>[2x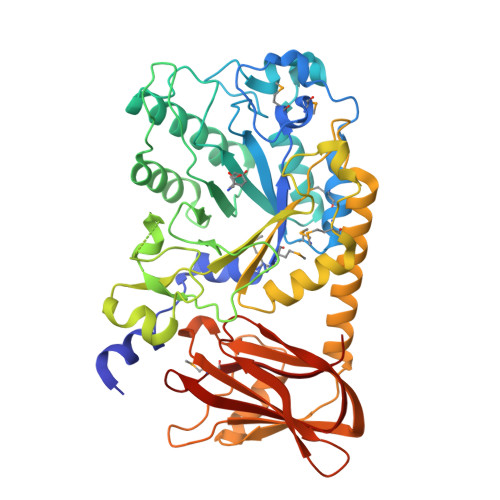]QGMNNPADAGINLNYLANVRPSSRQLAWQRMEMYAFLHFGMNTMTDREWGLGHEDPALFNPRNVDVDQWMDALVAGGMAGVILTCKHHDGFCLWPSRLTRHTVASSPWREGKGDLVREVSESARRHGLKFGVYLSPWDRTEESYGKGKAYDDFYVGQLTELLTQYGPIFSVWLDGANGEGKNGKTQYYDWDRYYNVIRSLQPDAVISVCGPDVRWAGNEAGHVRDNEWSVVPRRLRSAELTMEKSQQEDDASFATTVSSQDDDLGSREAVAGYGDNVCWYPAEVDTSIRPGWFYHQSEDDKVMSADQLFDLWLSAVGGNSSLLLNIPPSPEGLLAEPDVQSLKGLGRRVSEFREALASVRCEARTSSASAAAAHLVDGNRDTFWRPDADDAAPAITLTLPQPTTINAIVIEEAIEHGQRIEHLRVTGALPDGTERVLGQAGTVGYRRILRFDDVEVSSVTLHVDGSRLAPMISRAAAVRI[(2~{S},3~{S},4~{S},5~{R},6~{S})-6-[(2~{S})-3-butanoyloxy-2-heptanoyloxy-propoxy]-3,4,5-tris(oxidanyl)oxan-2-yl]methanesulfonic 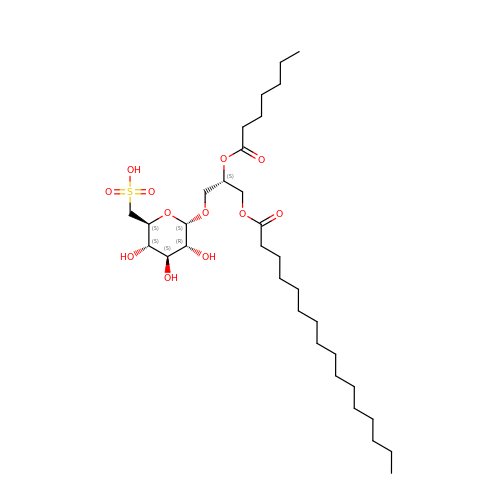acid | C32 H60 O12 S | IJGQUULJVRLGQW-CPYLTBOFSA-N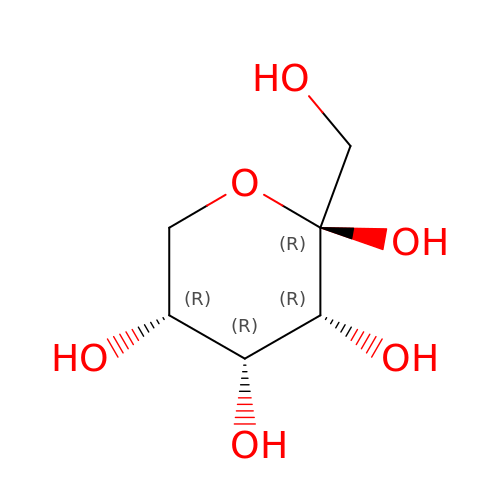D-Allulose | C6 H12 O6 | LKDRXBCSQODPBY-KVTDHHQDSA-N>AVEKYSLQGVVDGDKLLVVGFSEGSVNAYLYDGGETVKLNREPINSVLDPHYGVGRVILVRDVSKGAEQHALFKVNTSRPGEEQRLEAVKPMRILSGVDTGEAVVFTGATEDRVALYALDGGGLRELARLPGFGFVSDIRGDLIAGLGFFGGGRVSLFTSNLSSGGLRVFDSGEGSFSSASISPGMKVTAGLETAREARLVTVDPRDGSVEDLELPSKDFSSYRPTAITWLGYLPDGRLAVVARREGRSAVFIDGERVEAPQGNHGRVVLWRGKLVTSHTSLSTPPRIVSLPSGEPLLEGGLPEDLRRSIAGSRLVWVESFDGSRVPTYVLESGRAPTPGPTVVLVHGGPFAEDSDSWDTFAASLAAAGFHVVMPNYRGSTGYGEEWRLKIIGDPCGGELEDVSAAARWARESGLASELYIMGYSYG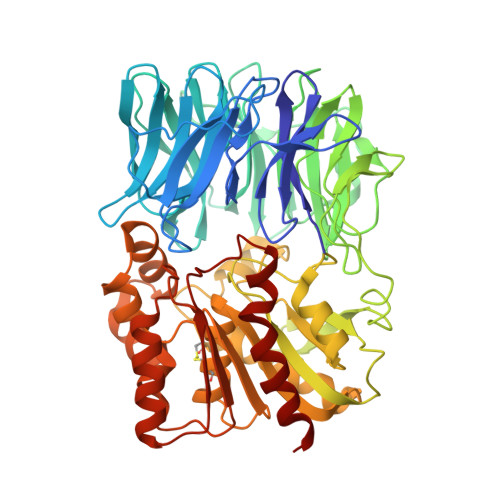GYMTLCALTMKPGLFKAGVAGASVVDWEEMYELSDAAFRNFIEQLTGGSREIMRSRSPINHVDRIKEPLALIHPQNDSRTPLKPLLRLMGELLARGKTFEAHIIPDAGHAINTMEDAVKILLPAVFFLATQRERR[2x]>MANIYKIDKLNNFNLNNHKTDDYSLCKDKDTALELTQKNIQKIYDYQQKLYAEKKEGLIIAFQAMDAAGKDGTIREVLKALAPQGVHEKPFKSPSSTELAHDYLWRVHNAVPEKGEITIFNRSHYEDVLIGKVKELYKFQNKADRIDENTVVDNRYEDIRNFEKYLYNNSVRIIKIFLNVSKKEQAERFLSRIEEPEKNWKFSDSDFEERVYWDKYQQAFEDAINATSTKDCPWYVVPADRKWYMRYVVSEIVVKTLEEMNPKYPTVTKETLERFEGYRTKLLEEYNYDLDTIRPIEKLEHHHHHH[4x]

EbPPK2 is a class III polyphosphate kinase that accepts a surprisingly broad range of substrates. PPKs catalyse the transfer of phosphate groups between adenosine-5′-triphosphate (ATP), as “energy currency” of the cell, and polyphosphate (polyP), a linear polymer of up to hundreds of phosphate units, as energy storage. While PPK2-I enzymes prefer the reaction from ADP to ATP, PPK2-II enzymes favour the reaction from AMP to ADP. The PPK2-III enzymes catalyse both aforementioned phosphorylation reactions, making this subclass the ideal source for enzymes used in ATP recycling or ATP analogue generation. The enzyme forms a homotetramer with four active sites and a polybasic patch which guides the polyP through a tunnel to the active site adjacent to the Walker A motif.

To better understand nucleobase recognition, we solved the first crystal structures of EbPPK2, both as a complex with polyP (2.3 Å) and as a ternary complex with polyP and the non-hydrolysable ATP analogue ACP (1.7 Å). In both EbPPK2 structures, the lid module covers the active site which includes the Walker A and Walker B motifs. From the opposite direction, a polyphosphate tunnel enables the entrance of polyP into the active site. The basic tunnel, also observed in other PPK2 structures, is defined by positively charged residues, namely K29, K70, R75, R188, R192, K198, K201, R241, K242 and R246. In the EbPPK2/polyP structure, polyP11 can be clearly resolved. The terminal phosphate of polyP protrudes into the active site and appears to be optimally positioned for the nucleophilic attack of the terminal phosphate of the nucleotide.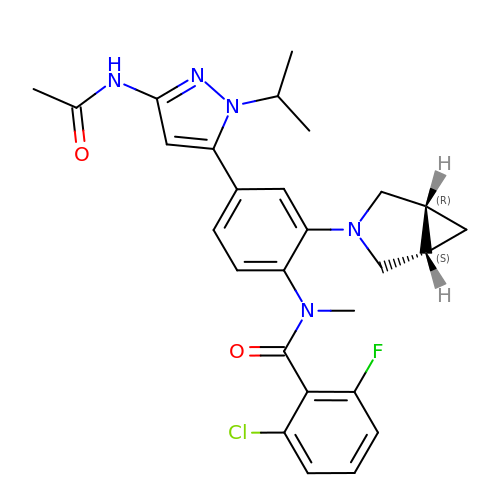N-{4-[3-(acetylamino)-1-(propan-2-yl)-1H-pyrazol-5-yl]-2-[(1R,5S)-3-azabicyclo[3.1.0]hex-3-yl]phenyl}-2-chloro-6-fluoro-N-methylbenzamide | C27 H29 Cl F N5 O2 | JGJWPIOGJPAGQE-KDURUIRLSA-N>[4x]MAKKTGAKYPKSLLSLPLVGSLPFLPRHGHMHNNFFKLQKKYGPIYSVR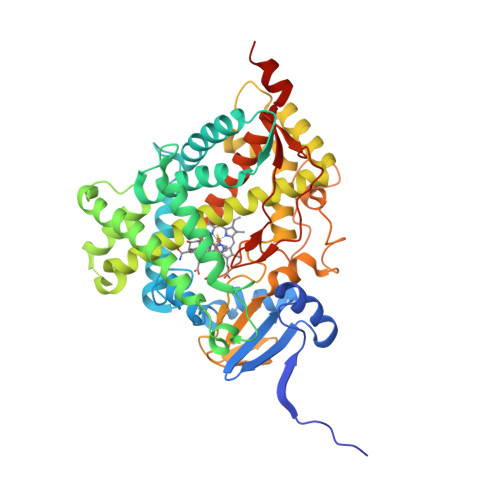MGTKTTVIVGHHQLAKEVLIKKGKDFSGRPQMATLDIASNNRKGIAFADSGAHWQLHRRLAMATFALFKDGDQKLEKIICQEISTLCDMLATHNGQSIDISFPVFVAVTNVISLICFNTSYKNGDPELNVIQNYNEGIIDNLSKDSLVDLVPWLKIFPNKTLEKLKSHVKIRNDLLNKILENYKEKFRSDSITNMLDTLMQAKMNSDNGNAGPDQDSELLSDNHILTTIGDIFGAGVETTTSVVKWTLAFLLHNPQVKKKLYEEIDQNVGFSRTPTISDRNRLLLLEATIREVLRLRPVAPMLIPHKANVDSSIGEFAVDKGTEVIINLWALHHNEKEWHQPDQFMPERFLNPAGTQLISPSVSYLPFGAGPRSCIGEILARQELFLIMAWLLQRFDLEVPDDGQLPSLEGIPKVVFLIDSFKVKIKVRQAWREAQAEGSTHHHH> AEAGITGTWYNQLGSTFIVTAGADGALTGTYESAVGNAES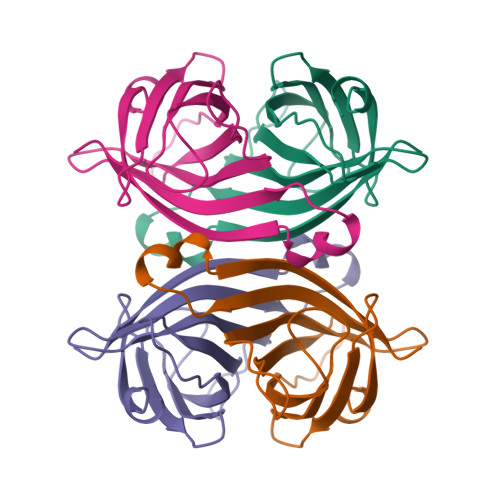RYVLTGRYDSAPATDGSGTALGWTVAWKNNYRNAHSATTWSGQYVGGAEARINTQWLLTSGTTEANAWKSTLVGHDTFTKV To date, all Ads display a characteristic, icosahedral symmetry in which 240 subunits of the trimeric hexon protein form the facets and 12 copies of the penton, comprising the pentameric penton base protein and the externally projecting trimeric fiber, form the vertices. At least in vitro and for most cell types, the fiber mediates the initial attachment to primary receptors, such as the D1 domain of the coxsackievirus and adenovirus receptor (CAR), sialic acids, CD46, and others (for review see Zhang & Bergelson). Our results showing that the CAV-2 fiber head contains a sialic acid binding site creates a paradox: both HAd37 and CAV-2 fiber heads contain CAR and sialic acid binding sites - but HAd37 uses sialic acid and CD46, while CAV-2 uses CAR (CAV-2 does not use CD46 to infect cells, unpublished data) to infect cells. We show by structural analysis that the CAV-2 fiber head also contains a sialic acid binding site, but in contrast to HAd37 this site is modestly involved in hemagglutination.

To address possible sialic acid binding via an alternative approach, we soaked CAV-2 fiber head crystals in solutions containing 2-3 sialyl-D-lactose. The crystal diffracted to 1.9 Å and the structure was solved by molecular replacement using our model of CAV-2 fiber head (crystallographic details are summarized in Table S1). The electron density maps showed clear density for six N-acetyl neuraminic acid (Neu5AC) moieties in the asymmetric unit, three per fiber head trimer. The density for the lactose moieties was weak, implying that these are flexible within the crystal. We found that the sialic acid binding site on CAV-2 head is distinct, both in sequence and location, from that found on the HAd37 fiber head. On the CAV-2 fibers head, sialic acid binds further away from the three-fold symmetry axis at the periphery of the trimer. The residues involved in binding (Asn435, Ser419, Ser416, Gln417 and Arg515) do not align with those involved in sialic acid-binding by HAd37 fiber head. All seven interactions between CAV-2 fiber head and sialic acid are hydrogen bonds or salt bridges, suggesting a relatively strong interaction compared to HAd37. Unlike HAd37 fiber head, no hydrophobic contacts contribute to sialic acid binding. Finally, sialic acid binds within a basic patch in each head.

>GAMSPPAAPITLWTGPGPSINGFINDTPVIRCFICLTRDSNLVTVNASFVGEGGYRIVSPTQSQFSLIMEFDQFGQLMSTGNINSTTTWGEKPWGNNTVQPRPSHTWKLCMPNREVYSTPAATISRCGLDSIAVDGAPSRSIDCMLIINKPKGVATYTLTFRFLNFNRLSGGTLFKTDVLTFTYVGENQ[6x]> VGVEDVGRFRLFDRHRLVELLPEGLAGELSRDVEMIPSATSPIGVMLRKATLELQMQLELFARVHAKSSADTRGETPLPRKRKETRKDGERDAREKKKDEGKDKDGGVGGRGLEEIGSRRSEDEWRERLSELRPFDARLAAVQRGFLLDGHRGVGKSCVLNYLIPWARENNWLVVYEPLPSRYAREIGDIKRSSAGVYIQSSFSQEFLERLGRFNRRLLEELPVARRCYGQAALDGVHRLYAERSYHSLLEKALEKDLDEIREQRDEELKRGSPHSGKDADLLDSQLREEILLARERLALWHTYRREVSIPSMKSRLPNPASVWEIAEFGLQNEAFATQALYEVWEQLKKQTQLNVLIAVDEWNECFPVSEYVSMRYEGTRFNGHI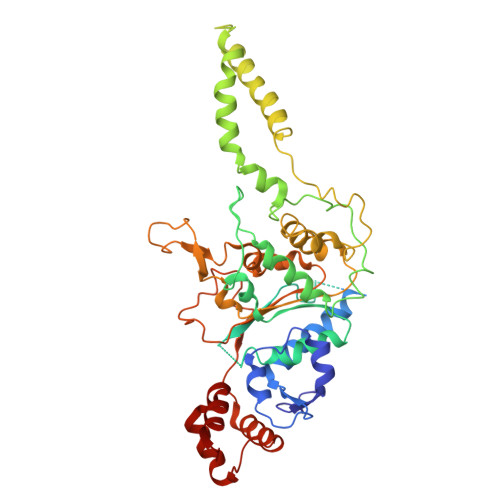PAFHLSTPRLLSRFDDAQQFQRGLKICATSWRRSNRRDYRPDLLGVRQEEIRTVRNFSPLEFANFVAYYHKKKILHEFPREKLDYFYMLSGGNGFQARRLLASLYGG> METNHITSLHHITICTGTAQGDIDFFVKVMGQRFVKRTLFYDGSIPIYHLYFADELGTPGTVMTTFPTRRTGQKGRKGSNQFTVCTYAIPKGSLEWWIGHLNAHGIATGEPGTRFGQRYVGFQHPDCGIDFEVLEDENDTRQPYDSPYVPIEHAQRGFHSWTASVRELEDMDFFMENCWNFEKIGEEGNRHRYRVKGTTESGTIIDLLHEPDRRQGSWTIAEGIIHHGAFAVPDMDIQARIKFETEGVGFTD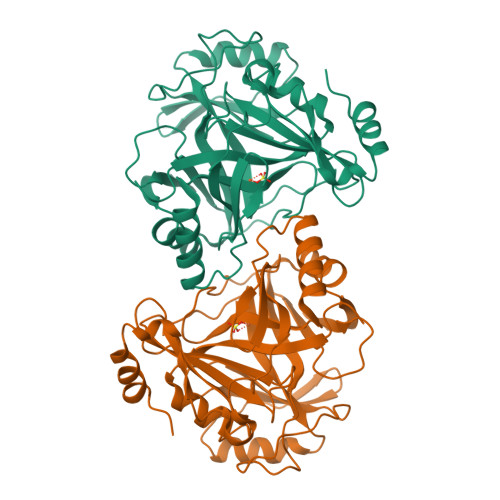FSDRKNRGYFESTYVRTPGGVMFEATHSLGFTHDEDERSLGMDLKVSPQFDDKKHLIEQAMEDDPIVV> GRHVRSYNHLQGDVRWRKLFSFTKYFLKIEKNGKVSGTKKENCPYSILEITSVEIGVVAVKAINSNYYLAMNKKGKLYGSKEFNNDCKLKERIEENGYNTYASFNWQHNGRQMYVALNGKGAPRRGQKT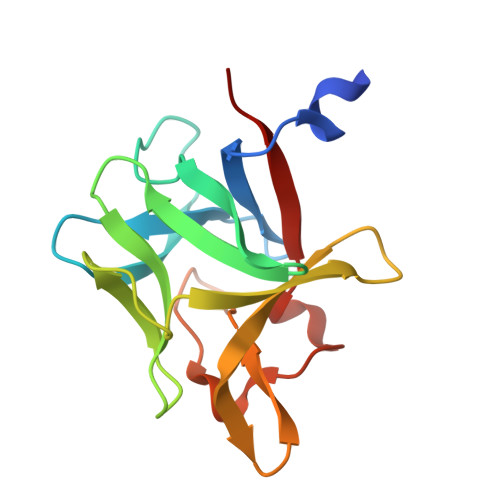RRKNTSAHFLPMVVHS> METGNKYIEKRAIDLSRERDPN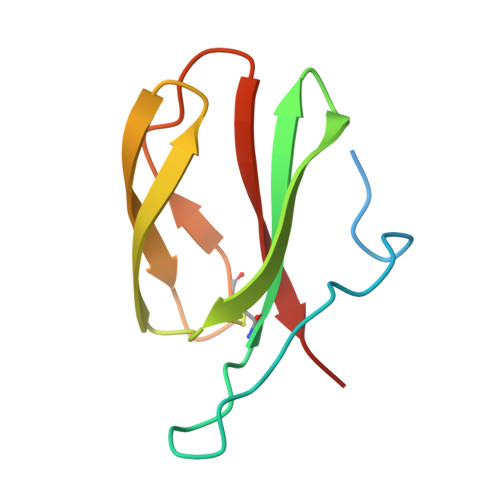FFDNPGIPVPECFWFMFKNNVRQDDGTCYSSWKMDMKVGPNWVHIKSDDNCNLSGDFPPGWIVLGKKRPGF>[2x]MRGSHHHHHHGSMPDLLTNVAENYVNQDLFAGIEWRIDQDGKPIFQGCAGVKDIETRTFIPKNAIYRIYSMTKPIVSFLAMMLIERGVFRLSSPIQNFDPRFKSMKVIDQHAHIEPATALITIEHLLTHQAGFSYDWSLGCPISAH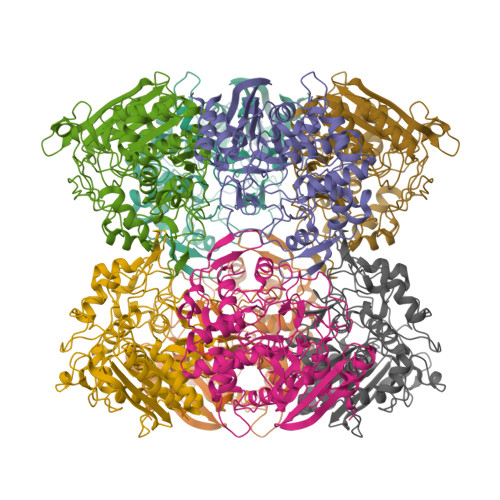YRDAQLIEDGGRDLTDMMGVLAELPLVFHPGTQWKYSISTDVLAHIIECATGERVDDLLQRLIFDPLDMQDTGFSLPLDGASRLMEVYGMRSLHGLPALKPAPHVLVPADLGSSHPTDDPDFRRGGHGLYSTLDDYMAFANMLLSGQTPEGETLLSPAVLKLALAPRVHFGARGMRINDEPFAGYSWNLLGRVMTDVGAAAYATHLGEFGWSGAAATYFWVDPTKNMTGCVMTQFLGSQHPIGSDMQAAAMSMLG>[2x]MQTTVTTMLLASVALAACAGGGSTPLPLPQQQPPQQEPPPPPVPLASRAACEALKDGNGDMVWPNAATVVEVAAWRDAAPATASAAALPEHCEVSGAIAKRTGIDGYPYEIKFRLRMPAEWNGRFFMEGGSGTNGSLSAATGSIGGGQIASALSRNFATIATDGGHDNAVNDNPDALGTVAFGLDPQARLDMGYNSYDQVTQAGKAAVARFYGRAADKSYFIGCSEGGREGMMLSQRFPSHYDGIVAGAPGYQLPKAGISGAWTTQSLAPAAVGLDAQGVPLINKSFSDADLHLLSQAILGTCDALDGLADGIVDNYRACQAAFDPATAANPANGQALQCVGAKTADCLSPVQVTAIKRAMAGPVNSAGTPLYNRWAWDAGMSGLSGTTYNQGWRSWWLGSFNSSANNAQRVSGFSARSWLVDFATPPEPMPMTQVAARMMKFDFDIDPLKIWATSGQFTQSSMDWHGATSTDLAAFRDRGGKMILYHGMSDAAFSALDTADYYERLGAAMPGAAGFARLFLVPGMNHCSGGPGTDRFDMLTPLVAWVERGEAPDQISAWSGTPGYFGVAARTRPLCPYPQIARYKGSGDINTEANFACAAPPLEHHHHHH

PETase cleaves BHET to MHET and EG, and the soluble MHET product is further hydrolyzed by MHETase to produce TPA and EG. Overall, the structure of MHETase is most similar to that of FAEs. The structural conservation between the hydrolase domains of MHETase and PETase is striking, and despite the large insertion of ∼240 residues representing the lid domain, residues Ser225, Asp492, and His528 effectively reconstitute the catalytic triad.

A similar Ca2+ binding site was characterized for Aspergillus oryzae FaeB (AoFaeB), wherein it was hypothesized to have a role in stabilizing the lid domain. To examine the effect of calcium binding, a fifth scenario absent of either MHET or Ca2+ was modeled in triplicate 150-ns simulations (the prior four scenarios each include bound Ca2+). These trajectories show evidence for lid stabilization upon Ca2+ binding mainly in the immediate vicinity of the calcium binding site. In fact, the terminal residues of the lid domain converge to within hydrogen-bonding distance of each other (Tyr252-Ala469, 2.9 Å), creating a compact linkage to the hydrolase domain. The lid domain of MHETase is exceptionally large, as average lid domains in α/β-hydrolases tend to be ∼100 residues, and is more typical of a lid from tannase family members (vide infra). One of the MHETase disulfides is located at the active site, connecting cysteines (Cys224 and Cys529) adjacent to the catalytic residues (Ser225 and His528, respectively), which is conserved in tannase family members.Within the last decade, OXA-48 has become one of the most widespread serine β-lactamases. This Ambler class D β-lactamase confers resistance toward penicillins and decreases susceptibility to our last-resort drugs, the carbapenems. However, it is a poor hydrolyzer of extended-spectrum cephalosporins, including ceftazidime. Over the course of 300 generations, we identified seven single variants of OXA-48 (L67F, P68S, F72L, F156C/V, L158P, and G160C).

To investigate substrate binding, all OXA-48 variants were crystalized and soaked with ceftazidime. We were able to solve the crystal structure of L67F to 1.9 Å with four chains (A to D) in the asymmetric unit (space group P212121), which were arranged into two dimers (chains A/C and B/D). Chain C and D carried a hydrolyzed ceftazidime molecule approximately 9 Å away from the active site S70. The R1-group of ceftazidime including the dihydrothiazine ring demonstrated clear electron density (2Fo-Fc); however, no electron density was observed for the R2-ring (top). Here, we found that Q98, R100, D101, W105, V120, P121, Q124, L158, T213, and R214 formed a cryptic pocket outside the active side and that these residues were involved in stabilizing the hydrolyzed ceftazidime molecule (top). D101, Q124, T213, and R214 were found to interact with ceftazidime via H-bonds. R214 was further involved in ionic interactions with two of the carboxylic acid groups of hydrolyzed ceftazidime. We found that K73 was carboxylated and that all first shell residues nicely aligned with the wild-type structure (middle). In the L67F variant, both with and without ceftazidime, L158 and I215 were shifted by 1 to 2 Å, respectively. While in the wild-type structure, the W221 side chain forms a water-mediated H-bond to the backbone nitrogen of M237, in L67F, W221 formed a H-bond to the main chain of F67.

>MRVLALSAVFLVASIIGMPAVAKEWQENKSWNAHFTEHKSQGVVVLWNENKQQGFTNNLKRANQAFFPASTFKIPNSLIALDLGVVKDEHQVFKWDGQTRDIATWNRDHNLITAMKYSVVPVYQEFARQIGEARMSKMLHAFDYGNEDISGNVDSFWLDGGIRISATEQISFLRKLYHNKLHVSERSQRIVKQAMLTEANGDYIIRAKTGYSTRIEPKIGWWVGWVELDDNVWFFAMNMDMPTSDGLGLRQAITKEVLKQEKIIP[4x]(2S)-2-{[(S)-[(3S)-3-amino-3-carboxypropyl](hydroxy)phosphoryl]methyl}pentanedioic 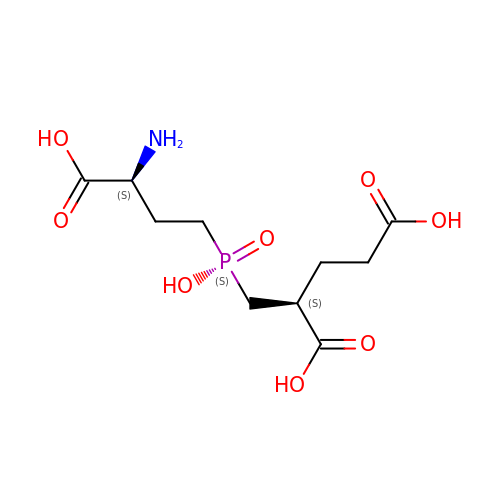acid | C10 H18 N O8 P | YLHAQDFYEKJARV-RQJHMYQMSA-N> AAGCUUUUGUGUCUUCAGCUUCCCUCUUCUCCUCGUGGGGUUCCGUUCCCGCGGUAGUGAGCCUGGUGUGGUUCCGCCCGCGCCAGUGAUGGAGGGUGCUUUAGGCACUAACAAGCUU

SL5 is the largest and most complex structural element in the 5′-proximal regions of βCoV RNA genomes. We further determined the 3D structures of the SL5 elements from these representatives using single-particle cryo-EM, which revealed remarkable structural similarity despite the low sequence conservation and variable lengths. All four structures exhibited a T-like shape, with the topology of the junctions featuring the SL5 basal stem positioned almost at right angles to the coaxial stack of SL5a/SL5b stems. Overall, the SL5 elements exhibited remarkable global structure conservation, despite the divergence at the level of individual nucleotide residues and their base pairs.

Cryo-EM single particle analyses generated high-quality 2D class averages and maps at 7.1, 6.5, 5.9, 6.6 Å overall resolutions for OC43-CoV, SARS-CoV-2, MERS-CoV, and RoBat-CoV, respectively. In subgenus D, SL5c is absent, causing SL5 to form a three-way junction (3WJ). The SL5 4WJ in OC43-CoV, SARS-CoV-2, MERS-CoV was formed by four canonical base pairs, coming from the four stems, while in RoBat-CoV the SL5 3WJ was formed by two canonical pairs and one G–U wobble pair. In RoBat-CoV RNA, unpaired nucleotides were present between the SL5 basal stem and SL5a (U170) and between the SL5 basal stem and SL5b (A231, U232). Nevertheless, the absence of SL5c in RoBat-CoV RNA had only a minor effect on the overall SL5 geometry. Distinct SL5 shapes were identified, such as the Y-shape in OC43-CoV, the more compact blob-like shape in MERS-CoV and SARS-CoV-2, and the rod-like shape in RoBat-CoV, in strong agreement with the cryo-EM maps of SL5. Notably, only for RoBat-CoV the Tm of the 5′-proximal region and the SL5 element differ by more than 2.5°C, indicating that the SL5 element of this representative exhibits lower thermal stability compared to the entire 5′-proximal region. MERS-CoV had the lowest Tm, while RoBat-CoV had the highest, likely due to its fewer single-stranded regions.>[4x]MELRAATKLTEEKYELKEGQTLDVKCDYTLEKFASSQKAWQIIRDGEMPKTLACTERPSKNSHPVQVGRIILEDYHDHGLLRVRMVNLQVEDSGLYQCVIYQP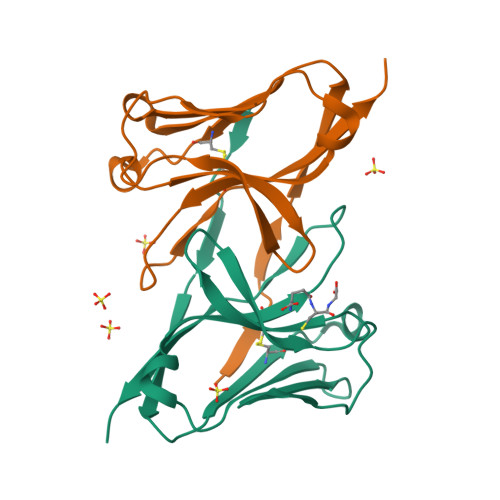PKEPHMLFDRIRLVVTLEHHHHHH>[2x]GPMGTDWPVYHRIDGPIVMIGFGSIGRGTLPLIERHFAFDRSKLVVIDPSDEARKLAEARGVRFIQQAVTRDNYRELLVPLLTAGPGQGFCVNLSVDTSSLDIMELARENGALYIDTVVEPWLGFYFDPDLKPEARSNYALRETVLAARRNKPGGTTAVSCCGANPGMVSWFVKQALVNLAADLGVTGEEPTTREEWARLAMDLGVKGIH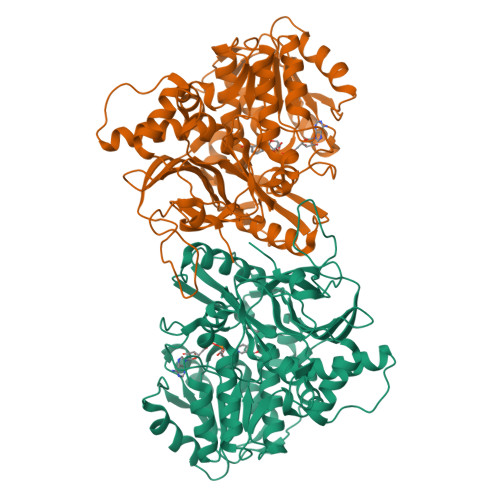IAERDTQRASFPKPFDVFVNTASVEGFVSEGLQPAELGWGTFERWMPDNARGHDSGCGAGIYLLQPGANTRVRSWTPTAMAQYGFLVTHNESISIADFLTVRDAAGQAVYRPTCHYAYHPCNDAVLSLHEMFGSGKRQSDWRILDETEIVDGIDELGVLLYGHGKNAYWYGSQLSIEETRRIAPDQNATGLQVSSAVLAGMVWALENPNAGIVEADDLDFRRCLEVQTPYLGPVVGVYTDWTPLAGRPGLFPEDIDTSDPWQFRNVLVRD> MESLPVIAAPSMWTRPQIKDFKEKIQQDADSVITVGRGEVVTVRVPTHEEGSYLFWEFATDNYDIGFGVYFEWTDSPNTAVSVHVSESSDDDEEEEENIGCEEKAKKNANKP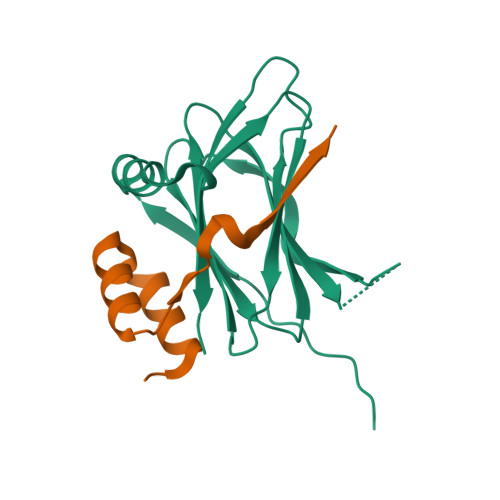LLDEIVPVYRRDCHEEVYAGSHQYPGRGVYLLKFDNSYSLWRSKSVYYRVYYTR;> GAMGPPQFKEIKISVAPDTPAPDAINDLLRSVDSQEVRDYCQKKGWIVIHPSNELVVEKHISR> SHMSFDKQNLIWIDLEMTGLDPEKERIIEIATIVTDKNLNILAEGPVLAVHQSDELLNKMNDWCQKTHSENGLIERIKASKLTERAAELQTLDFLKKWVP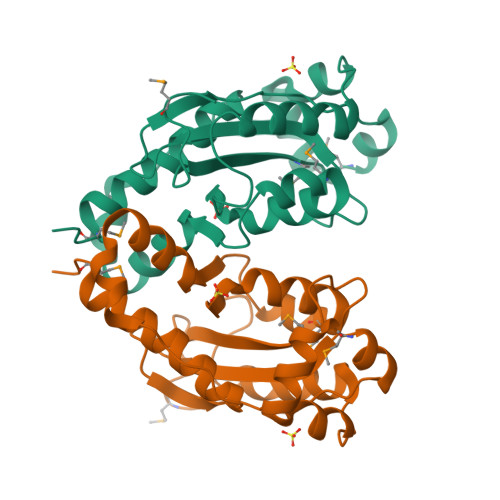KGASPICGNSIAQDKRFLVKYMPDLADYFHYRHLDVSTLKELAARWKPEILEGFKKENTHLALDDIRESIKELAYYREHFMKLD>[8x]GPHMSGSRKFFVGGNWKMNGSRDDNDKLLKLLSEAHFDDNTEVLIAPPSVFLHEIRKSLKKEIHVAAQNCYKVSKGAFTGEISPAMIRDIGCDWVILGHSERRNIFGESDELIAEKVQHALAEGLSVIACIGETLSERESNKTEEVCVRQLKAIANKIKSADEWKRVVVAYEPVWAIGTGKVATPQQAQEVHNFLRKWFKTNAPNGVDEKIRIIYGGSVTAANCKELAQQHDVDGFLVGGASLKPEFTEICKARQR

Helminth parasites are causal agents of diseases prevalent in humans. or TIM-barrel fold composed of 8 alternate β-strand and α-helices. three invariable catalytic residues (Lys, His, and Glu). enzymatic activity, leading to the concept that TPIs are obligated dimers.

helminths, we solved the crystal structures of TPIs from T. 2-PGA at 2.1 and 2.3 Å, respectively. in the presence of 2-PGA (TsTPI and SmTPI) and in its absence (OvTPI). and TsTPI exhibit a Tm of 75 and 57 ºC, respectively. interactions in SmTPI correlates with its higher melting point. illustrates the positions of residues TsTPI-S213 and SmTPI-S215. stabilize the SXD/E insert in SmTPI and TsTPI. TsTPI and SmTPI harbor 6 cysteine residues in their primary sequence. whereas only one thiol group is accessible in SmTPI at position C221. inhibited by targeting its solvent accessible cysteine.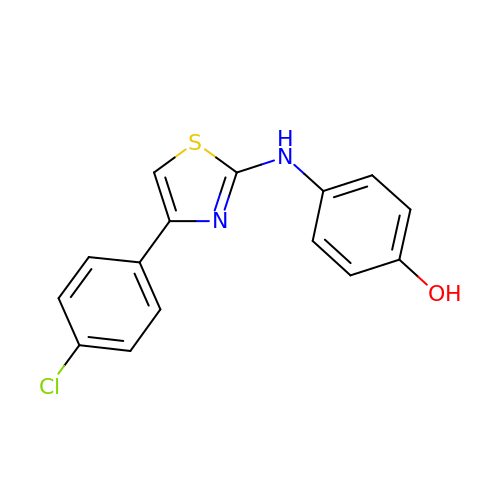4-{[4-(4-chlorophenyl)-1,3-thiazol-2-yl]amino}phenol | C15 H11 Cl N2 O S | ZFGXZJKLOFCECI-UHFFFAOYSA-N>MGSSHHHHHHSSGRENLYFQGHMATPAYMSITGTKQGLITAGAFTEDSVGNTYQEGHEDQVMVQGFNHEVIIPRDPQSGQPTGQRVHKPVVITKVFDKASPLLLAALTSGERLTKVEIQWYRTSAAGTQEH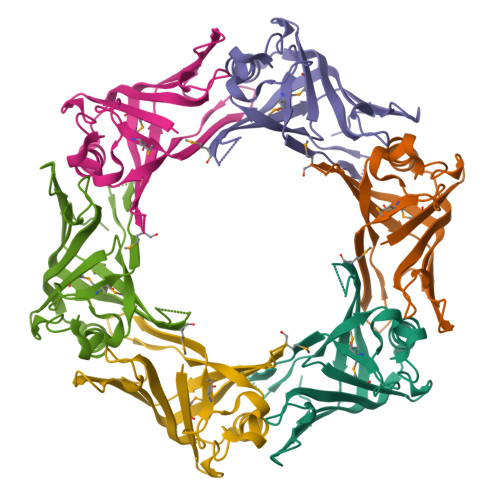YYTTVLEDAIIVDIKDYMHNCQDPGNAHFTHLEDVHFTYRKITWTHEVSGTSGSDDWRSPVAGS[6x]>ECVTQLLKDTCFEGGDITTVFTPSAKYCQVVCTYHPRCLLFTFTAESPSEDPTRWFTCVLKDSVTETLPRVNRTAAISGYSFKQCSHQISACNKDIYVDLDMKGINYNSSVAKSAQECQERCTDDVHCHFFTYATRQFPSLEHRNICLLKHTQTGTPTRITKLDKVVSGFSLKSCALSNLACIRDIFPNTVFADSNIDSVMAPDAFVCGRICTHHPGCLFFTFFSQEWPKESQRNLCLLKTSESGLPSTRIKKSKALSGFSLQSCRHSIPVFCHSSFYHDTDFLGEELDIVAAKSHEACQKL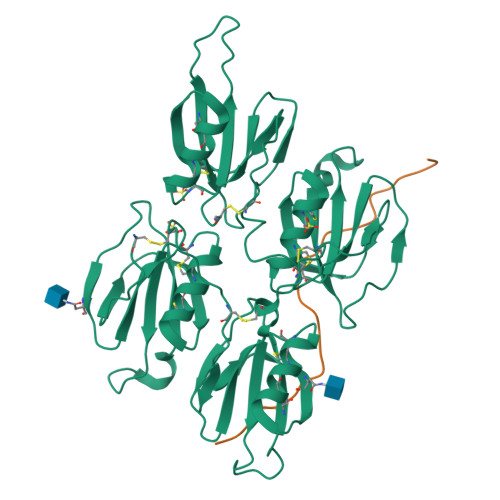CTNAVRCQFFTYTPAQASCNEGKGKCYLKLSSNGSPTKILHGRGGISGYTLRLCKM[2x];>SDDDWIPDIQIDPNGLSFNPISDFPDTTSPK[2x]> MKSSDIFHAYRYTPVFLKARQHDSGVNQYGLKPVNAYDFINPTNLVNFGRGTSFDNLGVRRAGRGEIDSSPSLGGSPVFTQAKLVGLSGEEQLTMCQSETMALRVCMARGGQDTCERESRALDACLS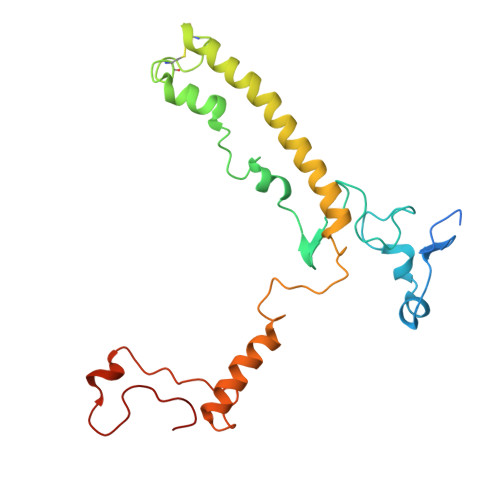RVGHLRRAMSEACGEFNDWFIQNVSDNHTKPFQHRPHDWRHFYAQEKLVRERQQNGHAYGRRPKQFSFGARYVKTEGYGKRPRLPYNK> MSLSKTFLNELANQALTNPNDFTKGEKKQESFLLEYVSANPTGPLHIGHARGAVFGDTLTRLARHLGYKFNTEYYVNDAGNQIYLLGLSILLSVKESILHENVEYPEQYYKGEYIVDLAKEAFEKFGKEFFSEENIPSLADWAKDKMLVLIKQNLEQAKIKIDSYVSERSYYDALNATLESLKEHKGIYEQEGKIWLASSQKGDEKDRVIIREDGRGTYLAADIVYHKDKMSRGYGKCINIWGADHHGYIPRMKAAMEFLGFDSNNLEIILAQMVSLLKDGEPYKMSKRAGNFIL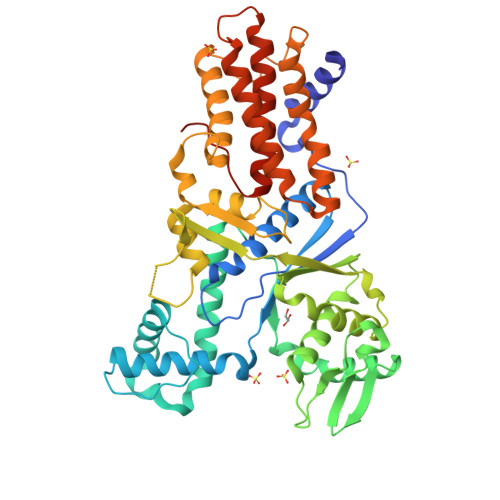MSDVVDEIGSDALRYIFLSKKCDTHLEFDISDLQKEDSSNPVYYINYAHARIHQVFAKAGKKIDDVMKADLQSLNQDGVNLLFEALNLKAVLNDAFEARALQKIPDYLKNLAANFHKFYNENKVVGSANENDLLKLFSLVALSIKTAFSLMGIEAKNKMEHEGHHHHHH> MAQHPPYCRNQPGKCQIPLRDLFDRAVVLSHYIHNLSSEMFSEFDKRYTHGRGFITKAINSCHTSSLATPEDKEQAQQMNQKDFLSLIVSILRSWNEPLYHLVTEVRGMQEAPEAILSKAVEIEEQTKRLLEGMELIVSQVH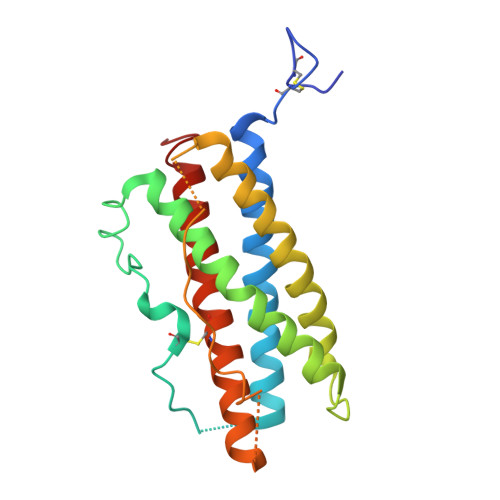PETKENEIYPVWSGLPSLQMADEESRLSAYYNLLHCLRRDSHKIDNYLKLLKCRIIHNNNC>NNPFYLRSSNSFQTLFENQNGRIRLLQRFNKRSPQLENLRDYRIVQFQSKPNTILLPHHADADFLLFVLSGRAILTLVNNDDRDSYNLHPGDAQRIPAGTTYYLVNPHDHQNLKIIKLAIPVNKPGRYDDFFLSSTQAQQSYLQGFSHNILETSFHSEFEEINRVLLGEEEEQRQQEGVIVELSKEQIRQLSRRAKSSSRKTISSEDEPFNLRSRNPIYSNNFGKFFEITPEKNPQLRDLDIFLSSVDINEGALLLPHFNSKAIVILVINEGDANIELVGIKEQQ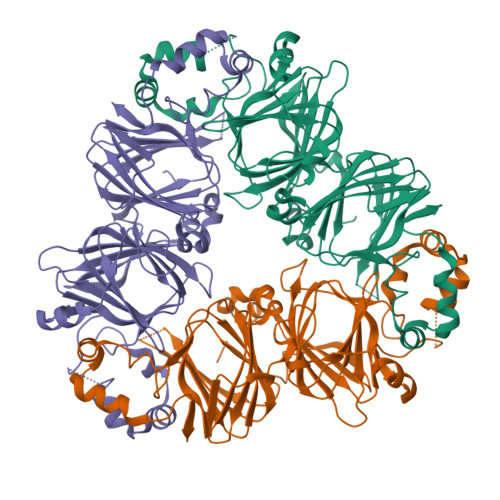QKQKQEEEPLEVQRYRAELSEDDVFVIPAAYPFVVNATSNLNFLAFGINAENNQRNFLAGEKDNVVRQIERQVQELAFPGSAQDVERLLKKQRESYFVDA[3x]> XPVGARGPAGPQGPRGDKGE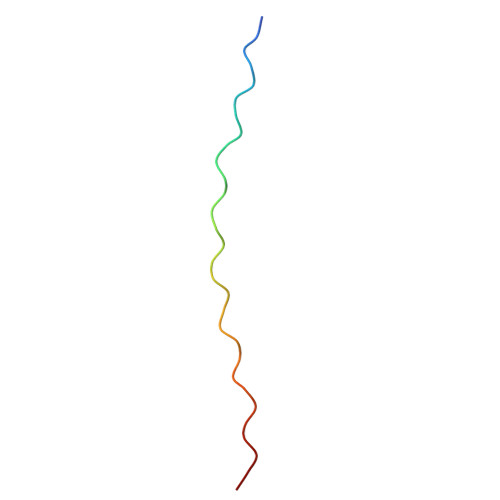TGEQGDRGIKG> MAHHHHHHVDDDDKMVHHDGFQTVKATIDWEHPMFKLYEKAKRNGKWNPADIDFSQDQKDFASLTSEEKISALPLVAGFSAGEEAVTLDILPMAHALARQGRLEDVLFLTT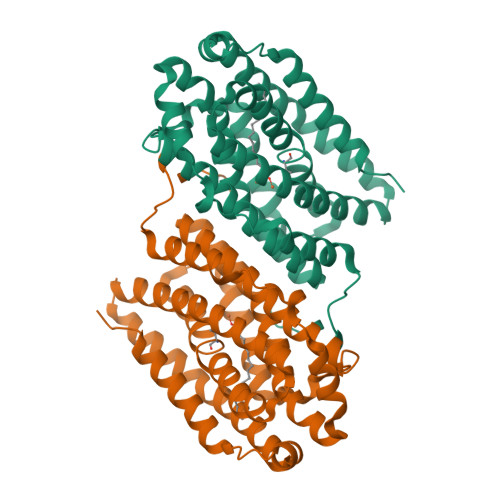FMHDEAKHVEMFSRWQQAVGIGQMDLSVFHNDHYKRIFYEALPEAMNRLYADDSPEAVIRAATVYNMIVAGTLAESGYYTFRQIYKKAGLFPGLLQGIDYLNMDEGRHIQFGIYTIQRIVNEDERYYELFIRYMDELWPHVIGYVDYLTELGKRQQQLARTYALEIDYDLLRHYVIKQFNLRKKQISRTKRVDVVEGLEKTAAES> GGACAUAUAAUCGCGUGGAUAUGGCACGCAAGUUUCUACCGGGC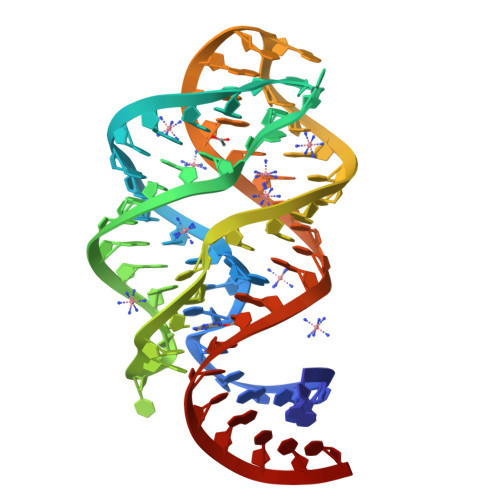ACCGUAAAUGUCCGACUAUGUCCA>[4x]MAEFRIAQDVVARENDRRASALKEDYEALGANLARRGVDIEAVTAKVEKFFVAVPSWGVGTGGTRFARFPGTGEPRGIFDKLDDCAVIQQLTRATP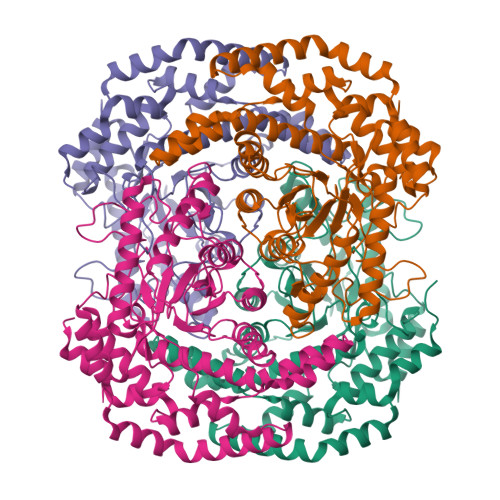NVSLHIPWDKADPKELKARGDALGLGFDAMNSNTFSDAPGQAHSYKYGSLSHTNAATRAQAVEHNLECIEIGKAIGSKALTVWIGDGSNFPGQSNFTRAFERYLSAMAEIYKGLPDDWKLFSEHKMYEPAFYSTVVQDWGTNYLIAQTLGPKAQCLVDLGHHAPNTNIEMIVARLIQFGKLGGFHFNDSKYGDDDLDAGAIEPYRLFLVFNELVDAEARGVKGFHPAHMIDQSHNVTDPIESLINSANEIRRAYAQALLVDRAALSGYQEDNDALMATETLKRAYRTDVEPILAEARRRTGGAVDPVATYRASGYRARVAAERPASVAGGGGIIGSHHHHHH> GAMGGA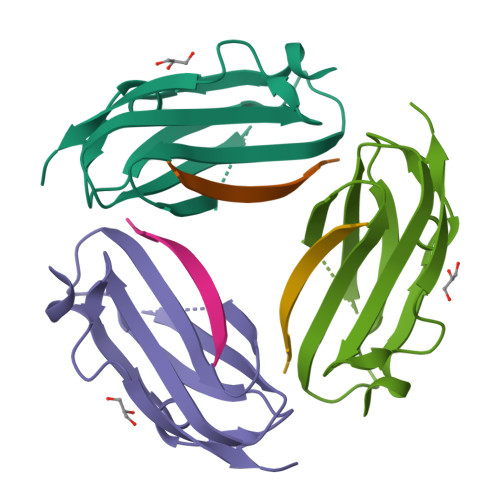HKVRAGGPGLERAEAGVPAEFSIWTREAGAGGLAIAVEGPSKAEISFEDRKDGSCGVAYVVQEPGDYEVSVKFNEEHIPDSPFVVPVASPS;> YRRFEKEKLKSQWNNDNPLFKSATTTVMNPKFAES>[6x]GAMGNQKTKASKL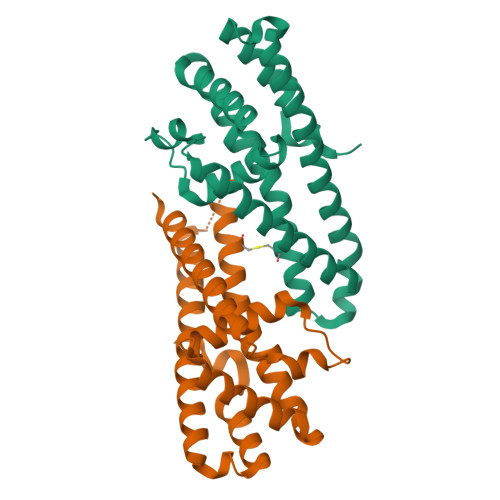ETAAKNLENQNKQEYIKINEIDAQGINFLATFKADEKDNLSQYEEMQIKRTIYSSLNYEKQKINTLKEILETLYNKLQHRYTSKEFIYQIVASIQYDIDRVLCLIKEAIIKDNLHTQNQKESELLMNLDSSLKTRQNFAKKLNETIDDYNKDSKNIQTNVDALATYMKENYKTLDSFKPIN> CGSMHSSGKDLNISLPLKT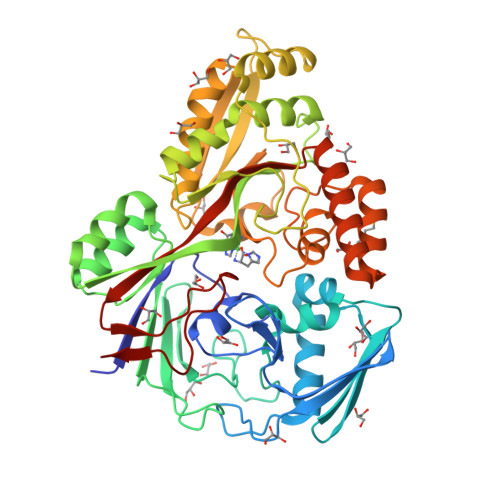KSIAPYETDVPVKIGAAESLFKTNDQGKIEKALVKSYHQPNDTTLDIELKDNIKFQNGQKLTAEKVKSSLENSMKKSDLVKYSLPISSITAKGQKLTIKTNSAYPELVSELANPFMAIYDTDAKSDVNQTPVGTGPYQIKDYKQSRKISLSNFKDYWQGKPKLDHITVTYQEDGNNRVRNLESQKDDLITDVPVNKVQDIENNQNLKVSKESGFRTSLLMYNHTNKKMTKSVREALDHIIDRQGIADHIYQGYAKPATSPFNDKIPYIKEPKLTKQNIEQAKMLLAKDGYTKEHPLKIKLITYDGRPELSKIAQVLQSDAKKANIEIDIKSVDDIEGYLKDRSAWDATMYSFGTIPRGDTGYFFNQAYKKDGAINKGDYNNSNVDDLINQLNHTVDVKERHNISNDIIKLSSRDVPNSYIAYNDQIVAANSKVKNYKVTPEGIYLIDYRTTIER> MAMPEKRPFERLPADVSPINYSLCLKPDLLDFTFEGKLEAAAQVRQATNQIVMNCADIDIITASYAPEGDEEIHATGFNYQNEDEKVTLSFPSTLQTGTGTLKIDFVGELNDKMKGFYRSKYTTPSGEVRYAAVTQFEATDARRAFPCWDEPAIKATFDISLVVPKDRVALSNMNVIDRKPYPDDENLVEVKFARTPVMSTYLVAFVVGEYDFVETRSKDGVCVRVYTPVGKAEQGKFALEVAAKTLPFYKDYFNVPYPLPKIDLIAIADFAAGAMENWGLVTYRETALLIDPKNSCSSSRQWVALVVGHELAHQWFGNLVTMEWWTHLWLNEGFASWIEYLCVDHCFPEYDIWTQFVSADYTRAQELDALDNSHPIEVSVGHPSEVDEIFDAISYSKGASVIRMLHDYIGDKDFKKGMNMYLTKFQQKNAATEDLWESLENASGKPIAAVMNTWTKQMGFPLIYVEAEQVEDDRLLRLSQKKFCAGGAYVGEDCPQWMVPITISTSEDPNQAKLKILMDKPEMNVVLKNVKPDQWVKLNLGTVGFYRTQYSSAMLESLLPGIRDLSLPPVDRLGLQNDLFSLARAGIISTVEVLKVMEAFVNEPNYTVWSDLSCNLGILSTLLSHTDFYEEIQEFVKDVFSPIGERLGWDPKPGEGHLDALLRGLVLGKLGKAGHKATLEEARRRFKDHVEGKQILSADLRSPVYLTVLKHGDGTTLDIMLKLHKQADMQEEKNRIERVLGATLLP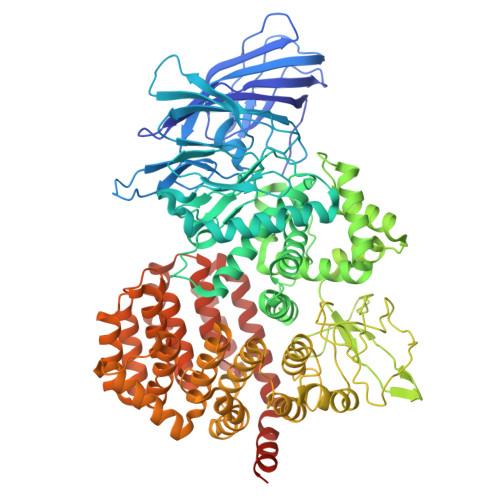DLIQKVLTFALSEEVRPQDTVSVIGGVAGGSKHGRKAAWKFIKDNWEELYNRYQGGFLISRLIKLSVEGFAVDKMAGEVKAFFESHPAPSAERTIQQCCENILLNAAWLKRDAESIHQYLLQRKASPPTVTGGLVPR> GSSHHHHHHLEVLFQGPVNALVSHLLVVEPEKLYAMPDPAGPDGHLPAVATLCDLFDREIVVTISWAKSIPGFSSLSLSDQMSVLQSVWMEVLVLGVAQRSLPLQDELAFAEDLVLDEEGARAAGLGELGAALLQLVRRLQALRLEREEYVLLKALALANSDSVHIEDAEAVEQLREALHEALLEYEAGRAGPGGGAERRRAGRLLLTLPLLRQTAGKVL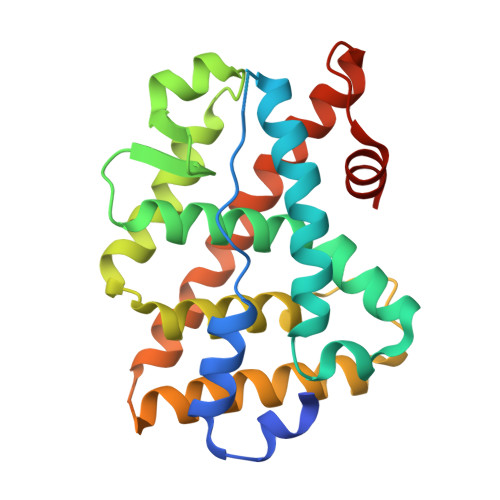AHFYGVKLEGKVPMHKLFLEMLEAMMD>[2x]MVTGGGAAPPGTVTEPLPSVIVLSAGRKMAAAAAAASGPGCSSAAGAGAAGVSEWLVLRDGCMHCDADGLHSLSYHPALNAILAVTSRGTIKVIDGTSGATLQASALSAKPGGQVKCQYISAVDKVIFVDDYAVGCRKDLNGILLLDTALQTPVSKQDDVVQLELPVTEAQQLLSACLEKVDISSTEGYDLFITQLKDGLKNTSHETAANHKVAKWATVTFHLPHHVLKSIASAIVNELKKINQNVAALPVASSVMDRLSYLLPSARPELGVGPGRSVDRSLMYSEANRRETFTSWPHVGYRWAQPDPMAQAGFYHQPASSGDDRAMCFTCSVCLVCWEPTDEPWSEHERHSPNCPFVKGEHTQNVPLSVTLATSPAQFPCTDGTDRISCFGSGSCPHFLAAATKRGKICIWDVSKLMKVHLKFEINAYDPAIVQQLILSGDPSSGVDSRRPTLAWLEDSSSCSDIPKLEGDSDDLLEDSDSEEHSRSDSVTGHTSQKEAMEVSLDITALSILQQPEKLQWEIVANVLEDTVKDLEELGANPCLTNSKSEKTKEKHQEQHNIPFPCLLAGGLLTYKSPATSPISSNSHRSLDGLSRTQGESISEQGSTDNESCTNSELNSPLVRRTLPVLLLYSIKESDEKAGKIFSQMNNIMSKSLHDDGFTVPQIIEMELDSQEQLLLQDPPVTYIQQFADAAANLTSPDSEKWNSVFPKPGTLVQCLRLPKFAEEENLCIDSITPCADGIHLLVGLRTCPVESLSAINQVEALNNLNKLNSALCNRRKGELESNLAVVNGANISVIQHESPADVQTPLIIQPEQRNVSGGYLVLYKMNYATRIVTLEEEPIKIQHIKDPQDTITSLILLPPDILDNREDDCEEPIEDMQLTSKNGFEREKTSDISTLGHLVITTQGGYVKILDLSNFEILAKVEPPKKEGTEEQDTFVSVIYCSGTDRLCACTKGGELHFLQIGGTCDDIDEADILVDGSLSKGIEPSSEGSKPLSNPSSPGISGVDLLVDQPFTLEILTSLVELTRFETLTPRFSATVPPCWVEVQQEQQQRRHPQHLHQQHHGDAAQHTRTWKLQTDSNSWDEHVFELVLPKACMVGHVDFKFVLNSNITNIPQIQVTLLKNKAPGLGKVNALNIEVEQNGKPSLVDLNEEMQHMDVEESQCLRLCPFLEDHKEDILCGPVWLASGLDLSGHAGMLTLTSPKLVKGMAGGKYRSFLIHVKAVNERGTEEICNGGMRPVVRLPSLKHQSNKGYSLASLLAKVAAGKEKSSNVKNENTSGTRKSENLRGCDLLQEVSVTIRRFKKTSISKERVQRCAMLQFSEFHEKLVNTLCRKTDDGQITEHAQSLVLDTLCWLAGVHSNGPGSSKEGNENLLSKTRKFLSDIVRVCFFEAGRSIAHKCARFLALCISNGKCDPCQPAFGPVLLKALLDNMSFLPAATTGGSVYWYFVLLNYVKDEDLAGCSTACASLLTAVSRQLQDRLTPMEALLQTRYGLYSSPFDPVLFDLEMSGSSCKNVYNSSIGVQSDEIDLSDVLSGNGKVSSCTAAEGSFTSLTGLLEVEPLHFTCVSTSDGTRIERDDAMSSFGVTPAVGGLSSGTVGEASTALSSAAQVALQSLSHAMASAEQQLQVLQEKQQQLLKLQQQKAKLEAKLHQTTAAAAAAASAVGPVHNSVPSNPVAAPGFFIHPSDVIPPTPKTTPLFMTPPLTPPNEAVSVVINAELAQLFPGSVIDPPAVNLAAHNKNSNKSRMNPLGSGLALAISHASHFLQPPPHQSIIIERMHSGARRFVTLDFGRPILLTDVLIPTCGDLASLSIDIWTLGEEVDGRRLVVATDISTHSLILHDLIPPPVCRFMKITVIGRYGSTNARAKIPLGFYYGHTYILPWESELKLMHDPLKGEGESANQPEIDQHLAMMVALQEDIQCRYNLACHRLETLLQSIDLPPLNSANNAQYFLRKPDKAVEEDSRVFSAYQDCIQLQLQLNLAHNAVQRLKVALGASRKMLSETSNPEDLIQTSSTEQLRTIIRYLLDTLLSLLHASNGHSVPAVLQSTFHAQACEELFKHLCISGTPKIRLHTGLLLVQLCGGERWWGQFLSNVLQELYNSEQLLIFPQDRVFMLLSCIGQRSLSNSGVLESLLNLLDNLLSPLQPQLPMHRRTEGVLDIPMISWVVMLVSRLLDYVATVEDEAAAAKKPLNGNQWSFINNNLHTQSLNRSSKGSSSLDRLYSRKIRKQLVHHKQQLNLLKAKQKALVEQMEKEKIQSNKGSSYKLLVEQAKLKQATSKHFKDLIRLRRTAEWSRSNLDTEVTTAKESPEIEPLPFTLAHERCISVVQKLVLFLLSMDFTCHADLLLFVCKVLARIANATRPTIHLCEIVNEPQLERLLLLLVGTDFNRGDISWGGAWAQYSLTCMLQDILAGELLAPVAAEAMEEGTVGDDVGATAGDSDDSLQQSSVQLLETIDEPLTHDITGAPPLSSLEKDKEIDLELLQDLMEVDIDPLDIDLEKDPLAAKVFKPISSTWYDYWGADYGTYNYNPYIGGLGIPVAKPPANTEKNGSQTVSVSVSQALDARLEVGLEQQAELMLKMMSTLEADSILQALTNTSPTLSQSPTGTDDSLLGGLQAANQTSQLIIQLSSVPMLNVCFNKLFSMLQVHHVQLESLLQLWLTLSLNSSSTGNKENGADIFLYNANRIPVISLNQASITSFLTVLAWYPNTLLRTWCLVLHSLTLMTNMQLNSGSSSAIGTQESTAHLLVSDPNLIHVLVKFLSGTSPHGTNQHSPQVGPTATQAMQEFLTRLQVHLSSTCPQIFSEFLLKLIHILSTERGAFQTGQGPLDAQVKLLEFTLEQNFEVVSVSTISAVIESVTFLVHHYITCSDKVMSRSGSDSSVGARACFGGLFANLIRPGDAKAVCGEMTRDQLMFDLLKLVNILVQLPLSGNREYSARVSVTTNTTDSVSDEEKVSGGKDGNGSSTSVQGSPAYVADLVLANQQIMSQILSALGLCNSSAMAMIIGASGLHLTKHENFHGGLDAISVGDGLFTILTTLSKKASTVHMMLQPILTYMACGYMGRQGSLATCQLSEPLLWFILRVLDTSDALKAFHDMGGVQLICNNMVTSTRAIVNTARSMVSTIMKFLDSGPNKAVDSTLKTRILASEPDNAEGIHNFAPLGTITSSSPTAQPAEVLLQATPPHRRARSAAWSYIFLPEEAWCDLTIHLPAAVLLKEIHIQPHLASLATCPSSVSVEVSADGVNMLPLSTPVVTSGLTYIKIQLVKAEVASAVCLRLHRPRDASTLGLSQIKLLGLTAFGTTSSATVNNPFLPSEDQVSKTSIGWLRLLHHCLTHISDLEGMMASAAAPTANLLQTCAALLMSPYCGMHSPNIEVVLVKIGLQSTRIGLKLIDILLRNCAASGSDPTDLNSPLLFGRLNGLSSDSTIDILYQLGTTQDPGTKDRIQALLKWVSDSARVAAMKRSGRMNYMCPNSSTVEYGLLMPSPSHLHCVAAILWHSYELLVEYDLPALLDQELFELLFNWSMSLPCNMVLKKAVDSLLCSMCHVHPNYFSLLMGWMGITPPPVQCHHRLSMTDDSKKQDLSSSLTDDSKNAQAPLALTESHLATLASSSQSPEAIKQLLDSGLPSLLVRSLASFCFSHISSSESIAQSIDISQDKLR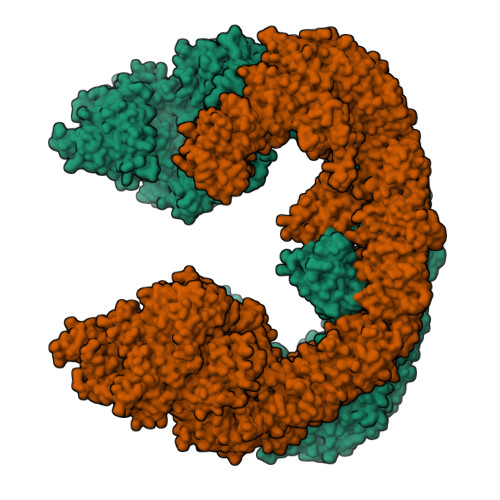RHHVPQQCNKMPITADLVAPILRFLTEVGNSHIMKDWLGGSEVNPLWTALLFLLCHSGSTSGSHNLGAQQTSARSASLSSAATTGLTTQQRTAIENATVAFFLQCISCHPNNQKLMAQVLCELFQTSPQRGNLPTSGNISGFIRRLFLQLMLEDEKVTMFLQSPCPLYKGRINATSHVIQHPMYGAGHKFRTLHLPVSTTLSDVLDRVSDTPSITAKLISEQKDDKEKKNHEEKEKVKAENGFQDNYSVVVASGLKSQSKRAVSATPPRPPSRRGRTIPDKIGSTSGAEAANKIITVPVFHLFHKLLAGQPLPAEMTLAQLLTLLYDRKLPQGYRSIDLTVKLGSRVITDPSLSKTDSYKRLHPEKDHGDLLASCPEDEALTPGDECMDGILDESLLETCPIQSPLQVFAGMGGLALIAERLPMLYPEVIQQVSAPVVTSTTQEKPKDSDQFEWVTIEQSGELVYEAPETVAAEPPPIKSAVQTMSPIPAHSLAAFGLFLRLPGYAEVLLKERKHAQCLLRLVLGVTDDGEGSHILQSPSANVLPTLPFHVLRSLFSTTPLTTDDGVLLRRMALEIGALHLILVCLSALSHHSPRVPNSSVNQTEPQVSSSHNPTSTEEQQLYWAKGTGFGTGSTASGWDVEQALTKQRLEEEHVTCLLQVLASYINPVSSAVNGEAQSSHETRGQNSNALPSVLLELLSQSCLIPAMSSYLRNDSVLDMARHVPLYRALLELLRAIASCAAMVPLLLPLSTENGEEEEEQSECQTSVGTLLAKMKTCVDTYTNRLRSKRENVKTGVKPDASDQEPEGLTLLVPDIQKTAEIVYAATTSLRQANQEKKLGEYSKKAAMKPKPLSVLKSLEEKYVAVMKKLQFDTFEMVSEDEDGKLGFKVNYHYMSQVKNANDANSAARARRLAQEAVTLSTSLPLSSSSSVFVRCDEERLDIMKVLITGPADTPYANGCFEFDVYFPQDYPSSPPLVNLETTGGHSVRFNPNLYNDGKVCLSILNTWHGRPEEKWNPQTSSFLQVLVSVQSLILVAEPYFNEPGYERSRGTPSGTQSSREYDGNIRQATVKWAMLEQIRNPSPCFKEVIHKHFYLKRVEIMAQCEEWIADIQQYSSDKRVGRTMSHHAAALKRHTAQLREELLKLPCPEGLDPDTDDAPEVCRATTGAEETLMHDQVKPSSSKELPSDFQLSAWSHPQFEK7-KETO-8-AMINOPELARGONIC ACID 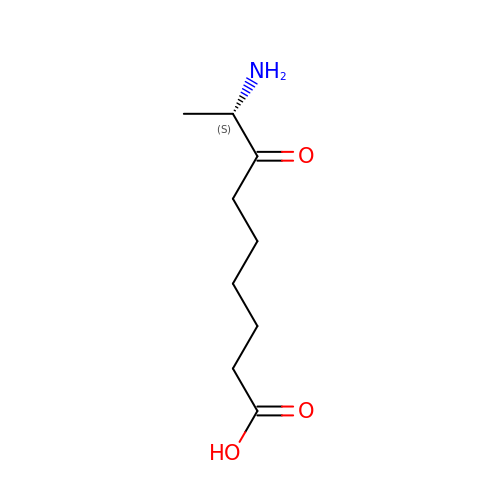| C9 H17 N O3 | GUAHPAJOXVYFON-ZETCQYMHSA-N>VAQISPQYPMFTVPLPIPPVKQPRLTVTNPVNGQEIWYYEVEIKPFTHQVYPDLGSADLVGYDGMSPGPTFQVPRGVETVVRFINNAEAPNSVHLHGSFSRAAFDGWAEDITEPGSFKDYYYPNRQSARTLWYHDHAMHITAENAYRGQAGLYMLTDPAEDALNLPSGYGEFDIPMILTSKQYTANGNLVTTNGELNSFWGDVIHVNGQPWPFKNVEPRKYRFRFLDAAVSRSFGLYFADTDAIDTRLPFKVIASDSGLLEHPADTSLLYISMAERYEVVFDFSDYAGKTIELRNLGGSIGGIGTDTDYDNTDKVMRFVVADDTTQPDTSVVPANLRDVPFPSPTTNTPRQFRFGRTGPTWTINGVAFADVQNRLLANVPVGTVERWELINAGNGFTHPIHIHLVDFKVISRTSGNNARTVMPYESGLKDVVWLGRRETVVVEAHYAPFPGVYMFHCHNLIHEDHDMMAAFNATVLPDYGYNATVFVDPMEELWQARPYELGEFQAQSGQFSVQAVTER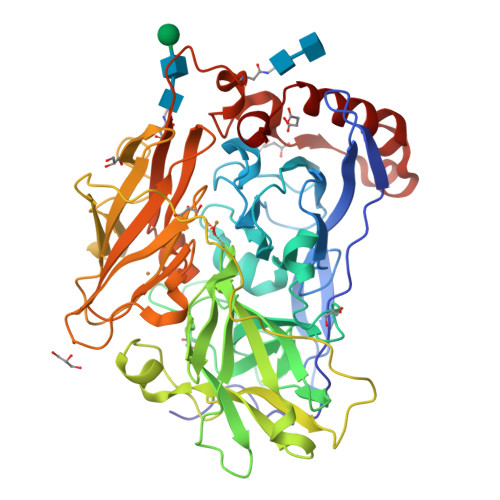IQTMAEYRPYAAADE[2x]> MKHHHHHHMKQNSPLDEENLTQENQDRGTHVDRGLASANVDFAFSLYKQLVLKAPDKNVIFSPLSISTALAFLSLGAHNTTLTEILKGLKFNLTETSEAEIHQSFQHLLRTLNQSSDELQLSMGNAMFVKEQLSLLDRFTEDAKRLYGSEAFATDFQDSAAAKKLINDYVKNGTRGKITDLIKDLDSQTMMVLVNYIFFKAKFEMPFDPQDTHQSRFYLSKKKYVMVPMMSLHHLTIPYFRDEELSCTVVQLNYTGNASALFILPDQDKMEEVEAMLSQETLSRFFESLEFREIGELYLPKFSISRDYNLNDILLQLGIEEAFTSKADLSGITGARNLAVSQVVHKAVLDVFEEGTERSAATALEVLFQ;> GPLVETRTIVRFNRPFLMI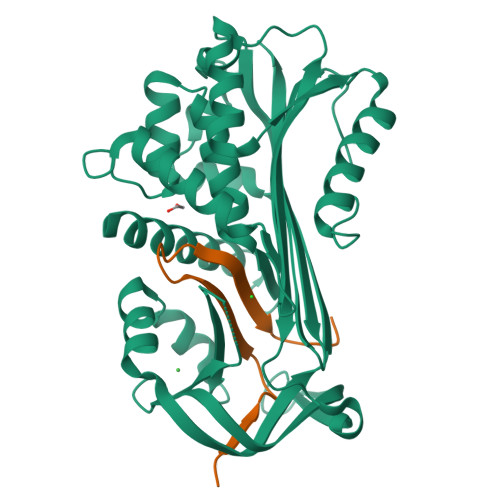IVDNFTWSIFFMSKVTNPKQA> ENLYFQSNAMVQIIFDSKTGNVQRFVNKTGFQQIRKVDEMDHVDTPFVLVTYTTNFGQVPASTQSFLEKYAHLLLGVAASGNKVWGDN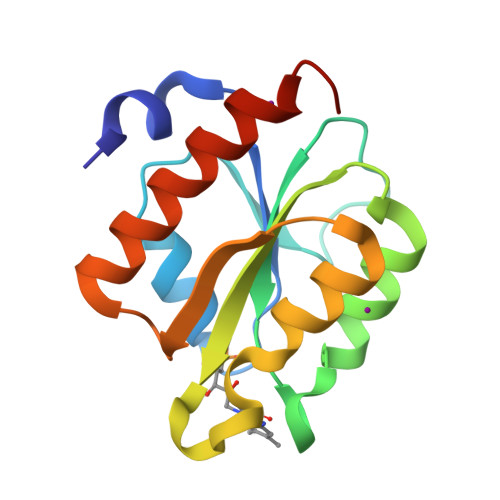FAKSADTISRQYQVPILHKFELSGTSKDVELFTQEVERVVTKSSAKMDPVK1,4-dimethylquinolin-2(1H)-one | C11 H11 N O | 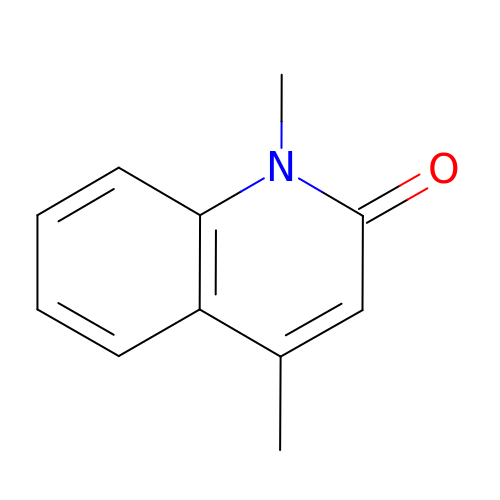CEONKCOBRZOYJS-UHFFFAOYSA-N> MLVVGSELQSDAQQLSAEAPRHGELQYLRQVEHILRCGFKKEDRTGTGTLSVFGMQARYSLRDEFPLLTTKRVFWKGVLEELLWFIKGSTNAKELSSKGVRIWDANGSRDFLDSLGFSARQEG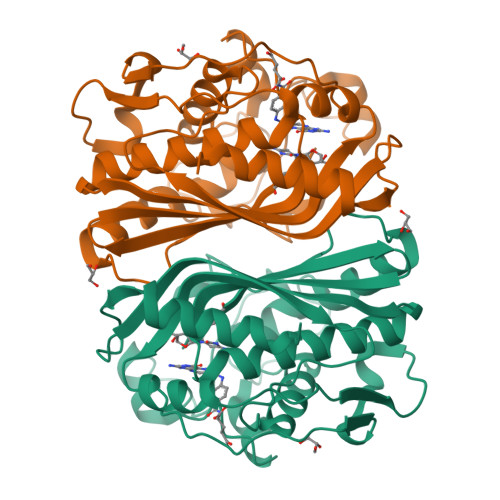DLGPVYGFQWRHFGAEYKDMDSDYSGQGVDQLQKVIDTIKTNPDDRRIIMCAWNPKDLPLMALPPCHALCQFYVVNGELSCQLYQRSGDMGLGVPFNIASYALLTYMIAHITGLQPGDFVHTLGDAHIYLNHIEPLKIQLQREPRPFPKLKILRKVETIDDFKVEDFQIEGYNPHPTIKMEMAV> MGSSHHHHHHGTGSYITSLYKKAGWMGSNEAQVKKESIGEIMGKLMQGEIGDEELSKRIKEIFGKRLQWGYKPTHQQQLAFNLDFIKSLKEMDMSGEIDTMNEETYELPSAFLEAAFGKTIKQSGCYFKDETTTIDEAEEASHELYCERAQIKDGQTVLDIGCGQGGLVLHIAQKYKNCHVTGLTNSKAQKNYILMQAEKLQLSNVDV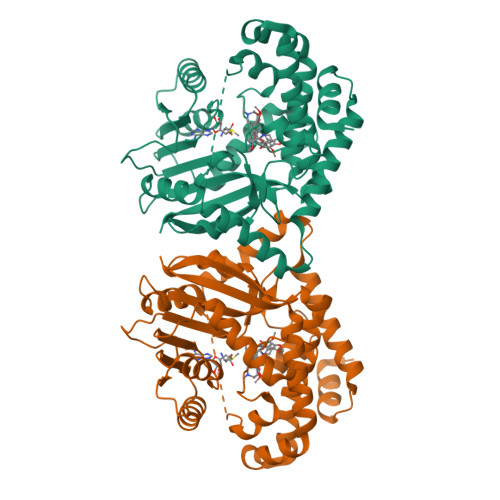ILADVTKHESDKTYDRILVIETIEHMKNIQLFMKKLSTWMTEDSLLFVDHICHKTFSHHFEAIDEDDWYSGFIFPKGCVTILSASALLYFQDDVTILDHWVVNGMHMARSVDAWRKKLDKNMELAREILLPGLGSKEAVNGVITHIRTFCMGGYEQFSYNNGEEWMVAQMLFKKK BAR protein endophilin B1 plays a key role in multiple cellular processes critical for oncogenesis, including autophagy and apoptosis. Endophilins are a highly conserved group of N-BAR proteins that contain an N-terminal amphipathic helix (H0) and a 20-residue amphipathic insert in helix 1 (H1i). These two motifs contribute to membrane association. BAR proteins are typically dimers in solution, where the dimer consists of three α-helices from each monomer that form a 6-helix bundle with a characteristic crescent shape.

Our EM structure of the endophilin B1 lipoprotein complex consists of six endophilin B1 dimers bound in two distinct conformations to a single artificial lipid platform. The final volume consisted of six endophilin B1 dimers and had a nominal resolution of 3.88 Å. Strong density could be observed for four dimers and slightly weaker density for two additional dimers. The volume contains a membrane bilayer density with anchored amphipathic helices. Interestingly, at higher contour levels the density corresponding to the membrane bilayer disappears, and where we expect to observe density corresponding to MSP2N2 scaffolds, there is none. Instead, we observe density that belongs to endophilin B1 amphipathic helices. Dimers bound to the surface of the bilayer and dimers that straddle the edges of the bicelle have distinct amphipathic helix conformations. The local resolution of the BAR domains is higher than that of the inserted amphipathic helices, suggesting the protein is flexible at the protein-lipid interface. Interestingly, no density corresponding to the SH3 domain-linker region is visible in any of our maps, either near the concave surface or proximal to the lateral part of the BAR domain.

>[12x]MNIMDFNVKKLAADAGTFLSRAVQFTEEKLGQAEKTELDAHLENLLSKAECTKIWTEKIMKQTEVLLQPNPNARIEEFVYEKLDRKAPSRINNPELLGQYMIDAGTEFGPGTAYGNALIKCGETQKRIGTADRELIQTSALNFLTPLRNFIEGDYKTIAKERKLLQNKRLDLDAAKTRLKKAKAAETRNSSEQELRITQSEFDRQAEITRLLLEGISSTHAHHLRCLNDFVEAQMTYYAQCYQYMLDLQKQLGSFPSNYLSNNNQTSVTPVPSVLPNAIGSSAMASTSGLVITSPSNLSDLKECSGSRKARVLYDYDAANSTELSLLADEVITVFSVVGMDSDWLMGERGNQKGKVPITYLELLN>MGSSHHHHHHSQDPMNSTAERMLS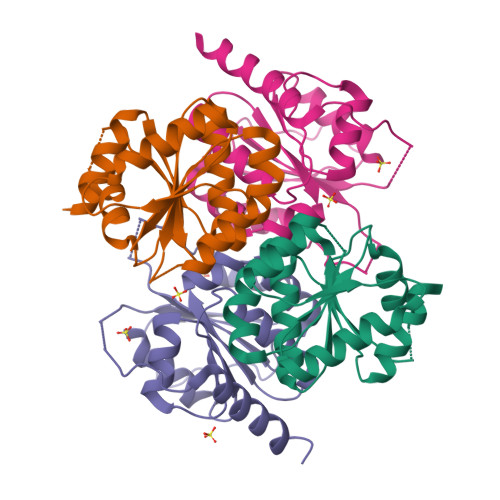TLTENNYTHFTGVPCSLLKGFFRLLESKEAIEKQNITFIPSIREDSALGVASGMYLGGRKCVMLMQNSGLGYCLNVLTSFNFIYDIPILLLISWRGAYGNDAVEHDIIGEKLTDLLDSVDIPYKELDYENSEGTILDALFLIEKTNRPVAILIKDEI[2x];>MNKHDAIQLILGQFPSAYLVSTCGHISRDLYNINDRARNFYMVGSMGMAAPVGLGLSTVYPDVPLVVLDGDGSFLMNMGIITMIGHQKPKNFIHVVLDNGMHESTGGQRTVPLVNVTDIALQVGYEYAIEINSGQKSFDLPNEGPGLIHIKVEPRSEKIGKRVHWTPQEIVQRFTNELTLENEVSV[2x]> SHMLRELCI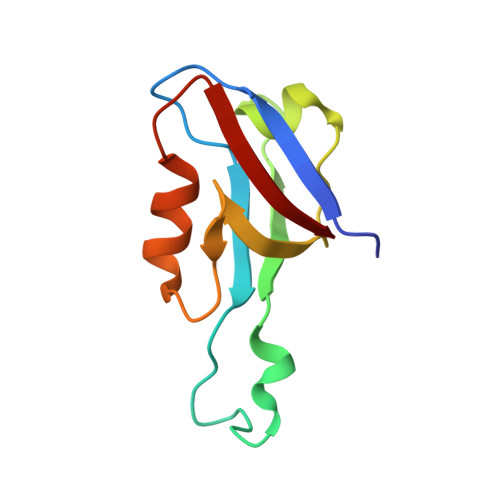QKAPGEGLGISIRGGARGHAGNPRDPTDEGIFISKVSPTGAAGRDGRLRVGLRLLEVNQQSLLGLTHGEAVQLLRSVGDTLTVLVC> MFGNKYEETPDVIGKSVKEAEQIFNKNNLKLGKISRSYSDKYPENEIIKTTPNTGERVERGDSVDVVISKGPEK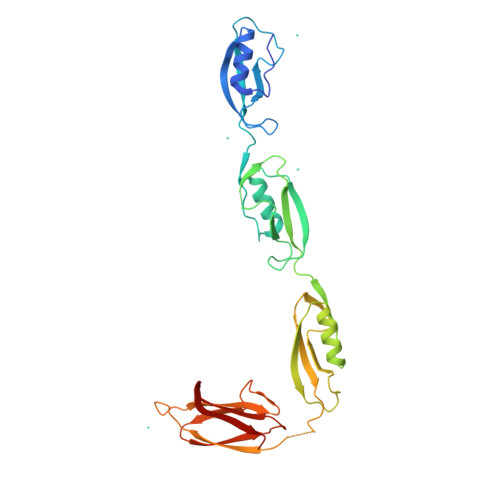VKMPNVIGLPKEEALQKLKSLGLKDVTIEKVYNNQAPKGYIANQSVTANTEIAIHDSNIKLYESLGIKQVYVEDFEHKSFSKAKKALEEKGFKVESKEEYSDDIDEGDVISQSPKGKSVDEGSTISFVVSKGKKSDSSDVKTTTESVDVPYTGKNDKSQKVKVYIKDKDNDGSTEKGSFDITSDQRIDIPLRIEKGKTASYIVKVDGKTVAEKEVSYDDI>[3x]PSETPQAEVGPTGCPHRSGPHSAKGSLEKGSPEDKEAKEPLWIRPDAPSRCTWQLGRPASESPHHHTAPAKSPKILPDILKKIGDTPMVRINKIGKKFGLKCELLAKCEFFNAGGSVKDRISLRMIEDAERDGTLKPGDTIIEPTSGNTGIGLALAAAVRGYRCIIVMPEKMSSEKVDVLRALGAEIVRTPTNARFDSPESHVGVAWRLKNEIPNSHILDQYRNASNPLAHYDTTAD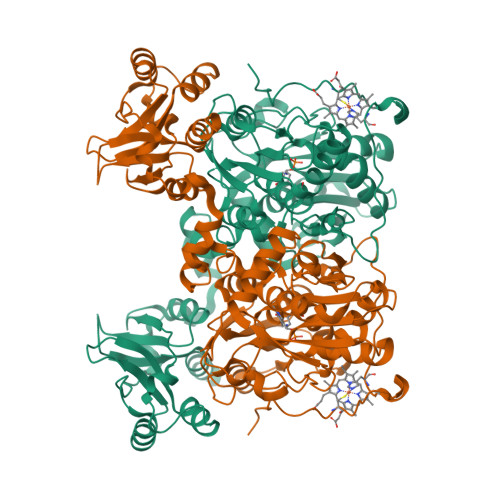EILQQCDGKLDMLVASVGTGGTITGIARKLKEKCPGCRIIGVDPEGSILAEPEELNQTEQTTYEVEGIGYDFIPTVLDRTVVDKWFKSNDEEAFTFARMLIAQEGLLCGGSAGSTVAVAVKAAQELQEGQRCVVILPDSVRNYMTKFLSDRWMLQKGFLKEEDLTEKKPWWWHLRVQELGLSAPLTVLPTITCGHTIEILREKGFDQAPVVDEAGVILGMVTLGNMLSSLLAGKVQPSDQVGKVIYKQFKQIRLTDTLGRLSHILEMDHFALVVHEQIQYHSTGKSSQRQMVFGVVTAIDLLNFVAAQERDQK Dye-decolourizing peroxidases (DyPs) are oxidative heme-containing enzymes that can oxidize organic substrates by first reacting with hydrogen peroxide to yield a catalytically active ferryl heme intermediate that results in electron transfer from substrates. The A-type DyP DtpAa from Streptomyces lividans has become a well characterized model system to investigate the mechanism of DyPs using a variety of techniques. This enzyme displays a typical DyP active site [Figs. 2(a) and 2(b)], with a heme coordinated on the proximal side by a histidine, whereas a solvent molecule is bound at the distal side. Complicating description and interpretation, the asymmetric unit of DtpAa crystals contains two molecules that show considerable differences in structure.

In view of the ∼1.6–1.8 Å distance of the two atoms, we propose the ligand to be either a ferric hydroperoxo intermediate (Fe–OOH−, also referred to as Compound 0), in line with previous investigations on chloroperoxidase, or a peroxo ligand. Importantly, the structures of the A and B molecules in the DtpAa dimer in the asymmetric unit differ in the conformation of the amino-acid stretch made up of residues 217–230 [Fig. 2(c)], which either lines up with the central β-sheet covering the distal side of the heme in the A molecule or is a loop bulging out of the active site (B molecule). Wilson plots calculated from the calculated intensities after the final stage of refinement are not affected by these complications; they solely reflect the falloff of Bragg diffraction with resolution (as the atomic model only accounts for this and not for other effects), and modern refinement programs calculate Icalc on an absolute scale. Icalc-based Wilson plots for the ID29 100 × 100 µm and the Cristallina-MX 100 × 100 µm data are shown in Fig. 12(b); a clear difference in the falloff of Bragg intensity with resolution is immediately apparent. To check that these are not spurious effects due to a difference in unit-cell parameters, we refined the 100 × 100 µm ID29 data using the 100 × 100 µm Cristallina-MX cell and found a change of only 0.03 Å in either parameter, much smaller than the effects seen with the actual data sets. Thus, the observed differences in the structures are not due to differences in unit-cell parameters but are due to radiation damage. Moreover, we observe an increase in the FeOOP displacement for the ID29-derived structures compared with those from the XFEL data, which is also much larger for the B molecule than for the A molecule. By comparing SFX and SSX data and the derived respective DtpAa structures, we see indications that local and global damage occurs at ID29 during the 90 µs exposure.

>[2x]GSAVPFHGAHQAGIATPVQDRLHFAAFDVTTEDRAAFVALLKEWTAAARRLTAGHAVGEGAYGGLPEAPPDDTGEALGLKPSRLTLTIGFGPSLFTRFGLADLRPEALADLPKFPGDNLDRARSGGDLCVQACADDPQVAVHAIRNLARIGFGKVVVRWSQLGFGKTSSTTPDKQTPRNLLGFKDGTRNIAGTEKDRLDRFVWAAEKDGTPWMTGGSYLVARRIRMHIETWDRASLQEQEDVFGRDKGEGAPVGKAKERDEPFLKAMKPDAHVRLAHPDSNGGATLLRRGYSFTDGTDGLGRLDAGLFFLAYQRDIRTGFVPVQRNLATDALNEYIQHVGSAVFAVPPGVRDADDWWGSTLFG> MAVLG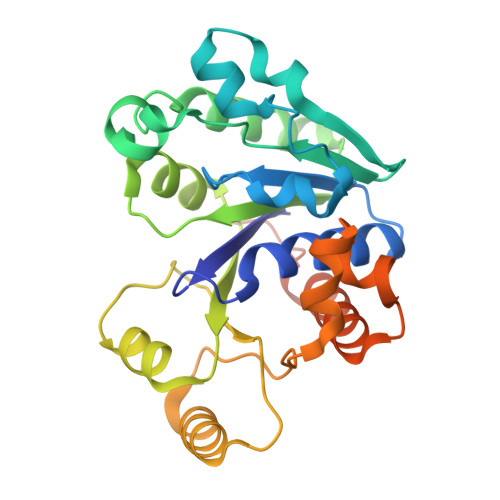LQGVRGGVGTTTITAALAWSLQMLGENVLVVDACPDNLLRLSFNVDFTHRQGWARAMLDGQDWRDAGLRYTSQLDLLPFGQLSIEEQENPQHWQTRLSDICSGLQQLKASGRYQWILIDLPRDASQITHQLLSLCDHSLAIVNVDANCHIRLHQQALPDGAHILINNFRIGSQVQDDIYQLWLQSQRRLLPMLIHRDEAMAECLAAKQPVGEYRSDALAAEEILTLANWCLLNYSGLKTPVGSKSAAALEHHHHHH>[2x]LDKLHVTSTRPQYVRIKNWGSGEILHDTLHHKATSCDFTCKSKSCLGSIMNPKSLTRGPRDKPTPLEELLPHAIEFINQYYGSFKEAKIEEHLARLEAVTKEIETTGTYQLTLDELIFATKMAWRNAPRCIGRIQWSNL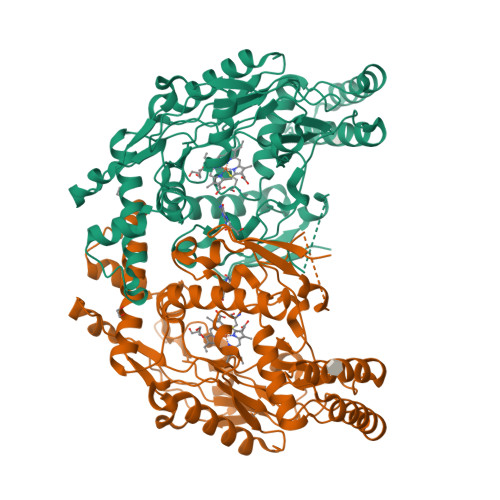QVFDARNCSTAQEMFQHICRHILYATNNGNIRSAITVFPQRSDGKHDFRLWNSQLIRYAGYQMPDGTIRGDAATLEFTQLCIDLGWKPRYGRFDVLPLVLQADGQDPEVFEIPPDLVLEVTMEHPKYEWFQELGLKWYALPAVANMLLEVGGLEFPACPFNGWYMGTEIGVRDFCDTQRYNILEEVGRRMGLETHTLASLWKDRAVTEINVAVLHSFQKQNVTIMDHHTASESFMKHMQNEYRARGGCPADWIALVPPVSGSITPVFHQEMLNYVLSPFYYYQIEPWKTHIWQNE> PQFHLWKRPVVTAHIEGQPVEVLLDTGA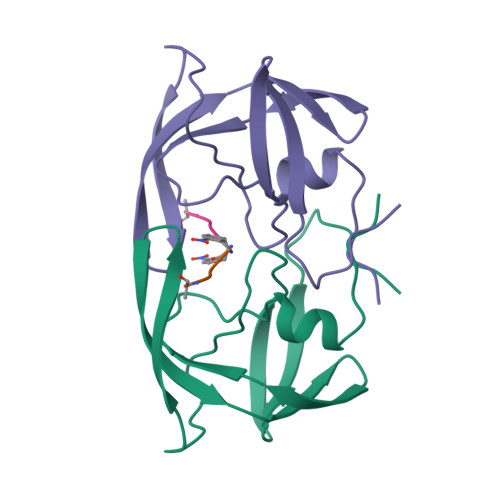DDSIVTGIELGPHYTPKIVGGIGGFINTKEYKNVEVEVLGKRIKGTIMTGDTPINIFGRNLLTALGMSLNF;> FEALS>[2x]SGSMEIR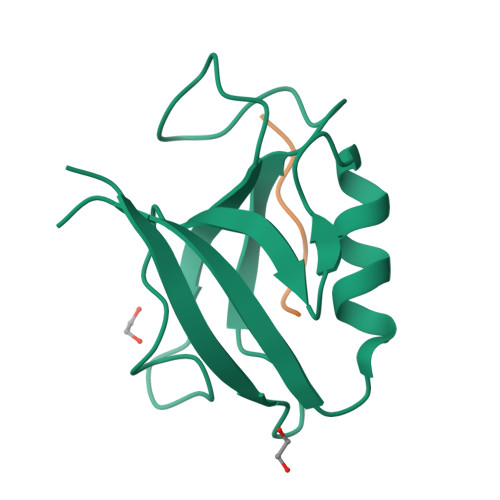VRVEKDPELGFRIAGGVGGRGNPFRPDDDGIFVTRVQPEGPASKLLQPGDKIIQANGYSFINIEHGQAISLLKTFQNTVELIIVREV;>YYESGWL[2x]> MLWKKSLSELRELLKRGEVSPKEVVESFYDRYNQTEEKVKAYITPLYGKALKQAESLKERELPLFGIPIAVKDNILVEGEKTTCASKILENFVAPYDATVIERLKKAGALIVGKTNLDEFAMGSSTEYSAFFPTKNPWDLERVPGGSSGGSAASVAVLSAPVSLGSDTGGSIRQPASFCGVIGIKPTYGRVSRYGLVAFASSLDQIGVFGRRTEDVALVLEVISGWDEKDSTSAKVPVPEWSEEVKKEVKGLKIGLPKEFFEYELQPQVKEAFENFIKELEKEGFEIKEVSLPHVKYSIPTYYIIAPSEASSNLAR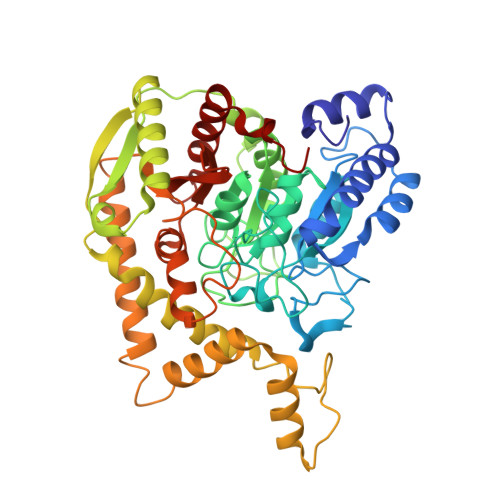YDGVRYGYRAKEYKDIFEMYARTRDEGFGPEVKRRIMLGTFALSAGYYDAYYLKAQKVRRLITNDFLKAFEEVDVIASPTTPTLPFKFGERLENPIEMYLSDILTVPANLAGLPAISIPIAWKDGLPVGGQLIGKHWDETTLLQISYLWEQKFKHYEKIPLT>PIKVIEQQQREMKNAEDNEKKDIQNIVKLKVFDQSIKTEDFYVIDVNSYCKANGDYLIGEFTVTQFSLQDGVKNSYHETIIPSCVPVGYMFDVKLGAEEFGLEMPGTDDAGPNYIQILANIIDYLKQKDRTVQVLPPMFTLPEKVDAVQNFISQMC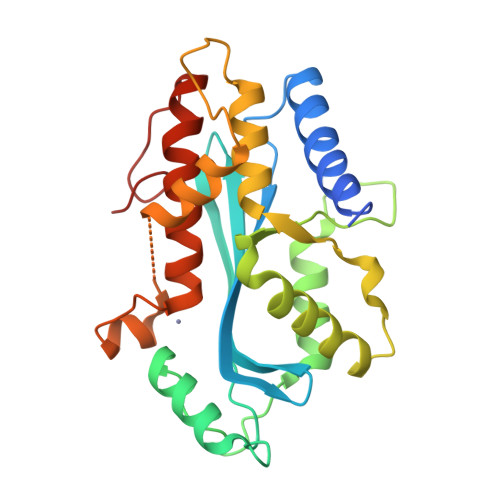NCATEDDSLFRIYKLDTFFFTLINAISSHHDEGFPKESLALTQLTKDLFDYTPGIACERHESLDKSNVCTTSRVKRWVFTILDRCCPLLGIPLQPGKHLPFDYDI[4x]> GGLEKDFLPLYFGWFLTKKSSETLRKAGQVFLEELGNHKAFKKELRHFISGDEPKEKLELVSYFGKRPPGVL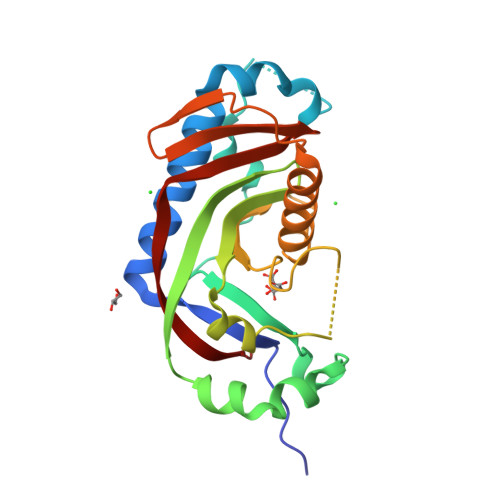HCATKFCDYGKAAGAEEYAQQEVVKRSYGKAFKLSISALFVTPKTAGAQVVLTDQELQLWPSDLDKPSASEGLPPGSRAHVTLGCAADVQPVQTGLDLLDILQQVKGGSQGEAVGELPRGKLYSLGKGRWMLSLTKKMEVKAIFTGYYG> MHHHHHHGTQQEALGMVETKGLTAAIEAADAMVKSANVMLVGYEKIGSGLVTVIVRGDVGAVK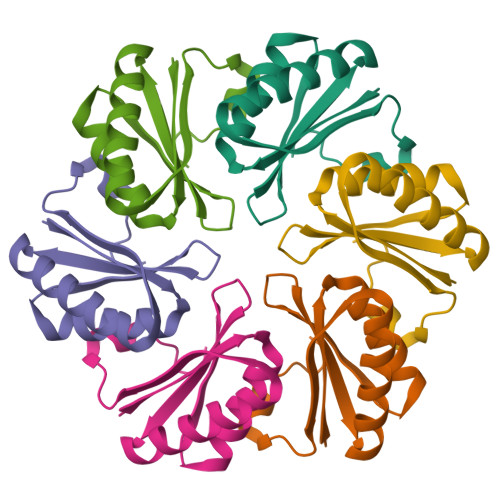AATDAGAAAARNVGEVKAVHVIPRPHTDVEKILPKGISQ>MADVVTEFGALTD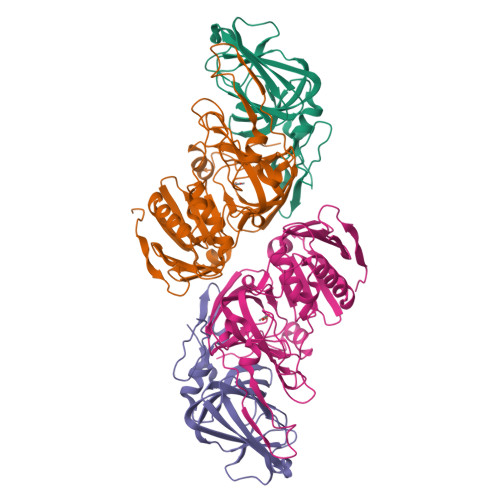YRKGGVEIIDDDPRNYVFSNVFEVAANAAPYERVAVGKNFEYVIESARAEGTSGWFSCAHDEFVLAMDGQIEVHLLKLDNSDAYVDPDSEGAVAIGEALPEGRKMGRIVLRRGHMALLPVGAAYRFYAEQPAAMLFQSIEGAVTVQKWGEICQTEAA[4x];>MAMSEALEIIDFGDSKARTDTEHLAINNETGYRSFRAGGFTFTRDEYFARLTWPGGSHIIPIDAFLRAMMRDVAWGFFYGVVNFDHVFGTINHYGEVTMFAGRFNDAYRNAGRDHEERFKSSALMAVFKDILSDWTVEGYDPFAAPMETGLPWGIKNGNNDEAISRQRVTARRMVGLPGDTPVRTDANGFPVNRQFADVPQEQPVVEAEPGFEAEVSAYNLFGYLSRSDVTWNPSVCSVVGDSLFCPTSEEFILPVEHGNDRCEWFLQLSDEIVWDVKDKESGKPRARVTARAGDICCMPADIRHQGYSTKRSMLLVWENGSPKIPQMIADGTAPVVPVTF[4x]>[6x]MTSAEMTSPNNNSEHQAIAKMRTMIEGFDDISHGGLPIGRSTLVSGTSGTGKTLFSIQFLYNGIIEFDEPGVFVTFEETPQDIIKNARSFGWDLAKLVDEGKLFILDASPDPEGQEVVGGFDLSALIERINYAIQKYRARRVSIDSVTSVFQQYDASSVVRRELFRLVARLKQIGATTVMTTERIEEYGPIARYGVEEFVSDNVVILRNVLEGERRRRTLEILKLRGTSHMKGEYPFTITDHGINIFPLGAMRLTQRSSNVRVSSGVVRLDEMCGGGFFKDSIILATGATGTGKTLLVSRFVENACANKERAILFAYEESRAQLLRNAYSWGMDFEEMERQNLLKIVCAYPESAGLEDHLQIIKSEINDFKPARIAIDSLSALARGVSNNAFRQFVIGVTGYAKQEEITGLFTNTSDQFMGAHSITDSHIEEITDTIILLQYVEIRGEMSRAINVFKMRGSWHDKAIREFMISDKGPDIKDSFRNFERIISGSPTRITVDEKSELSRIVRGVQEKGPESHHHHHH

A mixture of the KaiA, KaiB and KaiC proteins in the presence of ATP and Mg2+ exhibits stable oscillations in vitro between the hypo- and hyper-phosphorylated states of KaiC with a ∼24-h period. KaiC is a homo-hexamer that possesses auto-kinase, auto-phosphatase and ATPase activities. KaiC, a Ser-Thr kinase, contains two phosphorylation sites in the C-terminal (KaiCII) half, and harbors ATPase activity in the N-terminal (KaiCI) half. Phosphorylation of the S431 and T432 side chains in KaiCII follows a strict order such that a phosphate is first transferred to T432 and also first removed from T432; with the phosphorylation order represented by: TS→pTS→pTpS→TpS→TS.

Various mutants, including the KaiC T432E/S431E double mutant (KaiC-ee) have been designed to mimic the hyper-phosphorylated state of KaiC. Glutamate or asparate substitution of phosphorylation sites is a common approach to emulate the phosphorylated state of a protein. Glu, in particular, is spatially similar to both phosphorylated Thr and Ser, however Glu and Asp only contribute a single negative charge instead of the two negative charges of a phosphate group. To gain insight into the active site properties of the KaiC-ee mutant we determined its crystal structure at 3.0 Å resolution. Analysis of the region around the two introduced glutamates reveals several important changes compared to wt-KaiC. First, in the wt-KaiC structure both S431 and T432 are engaged in close contact with R393 from the same subunit, but neither E431 nor E432 are close to R393 in the KaiC-ee structure. The KaiC-ee mutant was designed to mimic a permanently phosphorylated form of KaiC that is unable to oscillate between the hypo- and hyper-phosphorylated states. However, the conformational changes observed in the structure of KaiC-ee and the presence of an additional phosphorylation site have to be taken into account when interpreting functional observations of this mutant. Therefore, the latest results indicate that the KaiC-ee mutant has a severely distorted in vivo rhythm. Despite the noted structural variations, the KaiC-ee mutant is clearly of use in biophysical studies and the changes in the overall structures between wt-KaiC and various phosphorylation mutants observed in the solid state (this work and [30]) and in solution are not dramatic.> 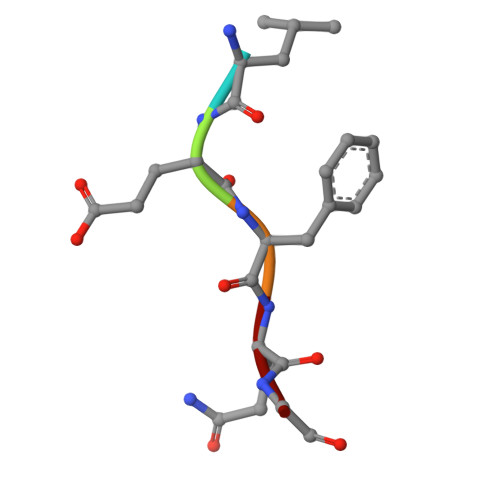LEFQG> MPFVNKQFNYKDPVNGVDIAYIKIPNVGQMQPVKAFKIHNKIWVIPERDTFTNPEEGDLNPPPEAKQVPVSYYDSTYLSTDNEKDNYLKGVTKLFERIYSTDLGRMLLTSIVRGIPFWGGSTIDTELKVIDTNCINVIQPDGSYRSEELNLVIIGPSADIIQFECKSFGHEVLNLTRNGYGSTQYIRFSPDFTFGFEESLEVDTNPLLGAGKFATDPAVTLAHELIHAGHRLYGIAINPNRVFKVNTNAYYEMSGLEVSFEELRTFGGHDAKFIDSLQENEFRLYYYNKFKDIASTLNKAKSIVGTTASLQYMKNVFKEKYLLSEDTSGKFSVDKLKFDKLYKMLTEIYTEDNFVKFFKVLNRKTYLNFDKAVFKINIVPKVNYTIYDGFNLRNTNLAANFNGQNTEINNMNFTKLKNFTGLFELEHHHHHH;> CA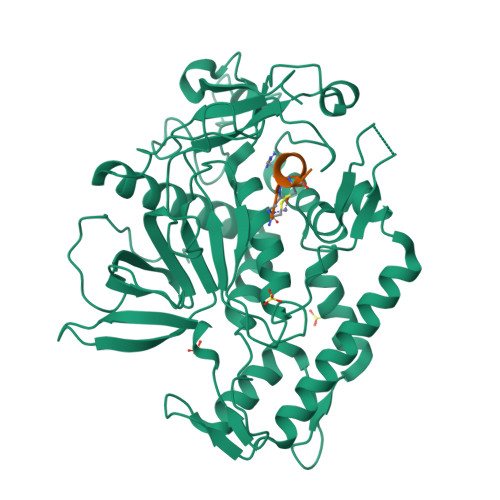RWTKCLX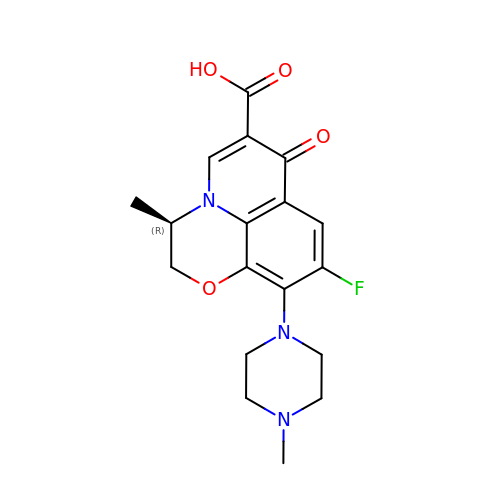DEXTROFLOXACINE | C18 H20 F N3 O4 | GSDSWSVVBLHKDQ-SNVBAGLBSA-N>[6x]MRGSHHHHHHMASMVDPRTPVIVGVGQFTERIDLDGYRGMSSVELATEAAKAALHDCGADADTVARAIDTVAGTRQFEISGPASAPLGVSSNYPRSVARNIGADPAHAVLEVIGGQSPQHLATEFGGKIAAGENDVVLIFGSENTSTLRHFSKAENKPDHSETVDGQLEDRGYGYDGIFDEYTIRHGLIGAPVQYGLLENARRARLGLSVADYRLAMAELFAPFSKVAAKNPYSSAPTERSVEELLTVTASNRMIVDPYPRLMVARDQVNQGAALLMMSVESARKLGVPEEKWVYLRGHADMKEPKLLERADIGASPASVTAVNEALRVAGIGLDDVAAFDLYSCFPFPVFNICDGTGLATDDPRGLTLTGGLPFFGGLGNNYSMHGIAEAVNEMRDKPGQFALVGANGGIASKYSVGIYSTEPADWVADNSAQLQAEHDAQPKVAITEKADGTGTIETYTVRYDWTPHTGIIIGRLDDGSRFLAKTKDEDLVKLLSEGDPIGAKIVVTPGEKSNRAVLA

Thiolases are a ubiquitous group of enzymes that are involved in biosynthetic and degradative pathways of lipid metabolism. In the last step of the β-oxidation pathway, degradative thiolases catalyze the shortening of the fatty acid chains by degrading 3-keto acyl CoA to form acetyl CoA and a shortened acyl CoA species. The protein encoded by one of the M. smegmatis thiolase-like genes (the thiolase-like protein type-1, MsTLP1) was over expressed in E. coli, purified and crystallized. A detailed analysis of the structure and biochemical properties of this protein revealed that its fold agrees with that of classical thiolase, but the nucleophilic active site cysteine and other characteristic thiolase sequence fingerprints are not conserved.

The crystal structure of MsTLP1 was determined using the single wavelength anomalous dispersion (SAD) method. The final R-factor and R-free of the refinement at 2.7 Å resolution are 23.3% and 26.1%, respectively. The polypeptide folds into two distinct domains: an N-terminal thiolase like domain (residues 1–407) and an additional C-terminal domain (residues 435–507), with a 27 residue long linker connecting the two domains. Thus, the N-terminal domain is organized into a five layered α/β/α/β/α structure characteristic of the thiolase superfamily. The C-terminal extra domain (residues 435–507) is made up of 6 β strands and resembles a barrel-like structure with three anti-parallel β-strands on either side of the barrel. Electron density is missing for four segments consisting of residues 17–25, 64–77, 135–170 and 253–254 in the thiolase domain as well as for the N-terminal hexa histidine tag. The six protomers in the asymmetric unit are related by a nearly perfect non-crystallographic 32 symmetry. Therefore, the hexameric state observed in the crystal structure of MsTLP1 is likely to be the result of crystal packing. Static Light Scattering (SLS) and size exclusion chromatography experiments show that, unlike other thiolases, MsTLP1 is a monomer of 56 kDa in solution. The most significant difference is that the active site nucleophilic cysteine, Cys89 of the CXS motif of Z. ramigera thiolase, has been replaced by Gly102 in MsTLP1.>MGSSHHHHHHAAPLPELLSNNGKHALMVDGAPYIILGSQTNNSSNYPDALKDVWPSMEKMGANTLSIPVAWEQIEPVEGQFDFSFVDVLLKEARQRKVRLVLLWFATWKNNAPHYAPAWVKLDNARFPRVVKEDGDTLNSLSPLGQNTLAADKKAFVELMKYLAKRDKDHTVIMVQVQNEVGTYGAVRDYSPMAQAVFNAAVPDDLIQKLQLKPGTWSQVFGRDADEFFHAYQIARYCDEVTVAGKAIKNLPMYVNVALRNPFNPGLPGQYSSGGGTDNVLHIWKAAAPNIDLIAPDIYFRDYKTVSKVLELYTRPDNALFVAEIGNDQPFARYLFPTLGKGGIGFSPFGMDDTDYTNYPLGAKVYNDETIEQFAQVYRLVNPMMREWARLSYQGQVWGVAEPLDSTTETQKIWNAEATPEEKEQHKKDRASALTQQLDLGLWDAEVTYGRPMFWVTPPEGNTPAAGGALIAQLDDNEYLVTAYKARVEFKPSQELAGKKFMIERVEEGRFEKGKWVMERVWNGDQTDWG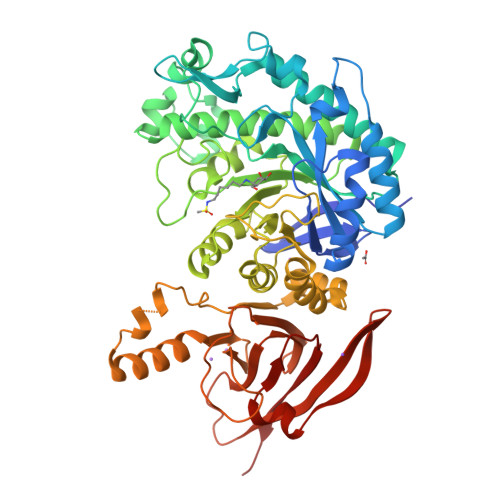LNFTDRPHLLRVKMASYSVQ[8x]> MTVRKNQATLTADEKRRFVAAVLELKRSGRYDEFVRTHNEFIMSDTDSGERTGHRSPSFLPWFRRFLLDFEQALQSVDSSVTLPYWDWSADRTVRASLWAPDFLGGTGRSTDGRVMDGPFAASTGNWPINVRVDSRTYLRRSLGGSVAELPTRAEVESVLAISAYDLPPYNSASEGFRNHLEGWRGVNLHNRVHVWVGGQMATGVSPNDPVFWLHHAYVDKLWAE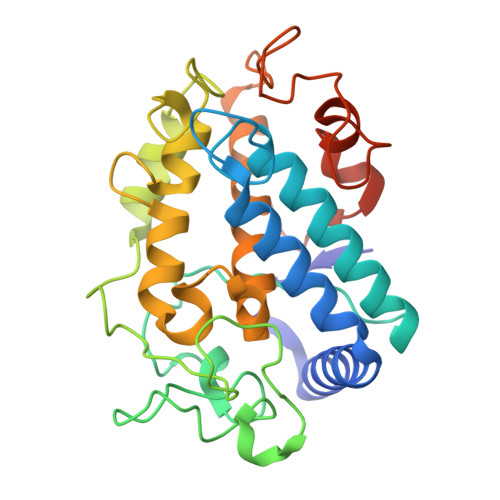WQRRHPDSAYVPTGGTPDVVDLNETMKPWNTVRPADLLDHTAYYTFDALEHHHHHH Sdk1 and Sdk2 are single-pass transmembrane proteins, with extracellular regions composed of 6 N-terminal immunoglobulin (Ig) domains followed by 13 fibronectin type III (FNIII) domains, and a relatively short intracellular domain terminating in a Postsynaptic density/Discs Large/ZO-1 (PDZ) binding motif. Here, we report the crystal structures of cell-cell adhesive homophilic dimers of mouse Sdk1 and Sdk2, each mediated by the four N-terminal Ig domains. These four domains adopt a horseshoe conformation, like many other IgSF cell-cell recognition proteins, but they interact in a unique back-to-back anti-parallel manner not previously observed. Overall, our data suggest a model in which Sdks form cis dimers on isolated cell surfaces, which dissociate to form trans dimers through the same interface when contact is made to a cell surface expressing the cognate Sdk.

The Ig1:Ig1 interface, for both Sdk1 and Sdk2, is centered on N22, which hydrogen bonds with the main chain of R23, and is supported by interactions between hydrophobic residues (L19, V25). Mutating residues in the central Ig1:Ig1 interface (N22R in Sdk1 and N22R, N22S and H18R/N22S in Sdk2) resulted in the loss of dimerization for both Sdk1 and Sdk2 in AUC experiments. These results—particularly the Sdk2 N22S mutation—highlight the critical importance of N22 and the two hydrogen bonds it forms to the dimer interaction. Consistent with this, a crystal structure of Sdk2Ig1–4 H18R/N22S showed a loss of the back-to-back dimer interaction. The Ig1–2 interface mutants (Sdk1 N22R and Sdk2 H18R/N22S) showed a loss of both homophilic and heterophilic binding revealing that the heterophilic interaction observed here is mediated by the same interface as the homophilic interaction.

>GPAGAQDDVPPYFKTEPVRTQVRLEGSRLVLTCMAEGSWPLEFKWLHNNRELTRFSLEYRYMITSLDRTHAGFYRCIVRNRMGALLQRQTEVQVAYMGSFEEGEKRQSVNHGEAAVIRAPRISSFPRPQVTWFRDGRKIPPSSRIAITLENTLVILSTVAPDAGRYYVQAVNDKNGDNKTSQPITLAVENVGGPADPIAPTIIIPPKNTSVVAGTSEVTMECVANARPLIKLHIVWKKDGAPLSSGISDYNRRLTIANPTVSDAGYYECEAMLRSSSVAPVTRGAYLSVLEPPQFVREPERHITAEMEKVVDIPCRAKGVPPPSITWYKDAALVEVGKLTRFKQRSDGGLQISGLLPDDTGMLQCFAHNAAGEAQTSTYLAVTS[4x]> IVGGYTCGANTVPYQVSL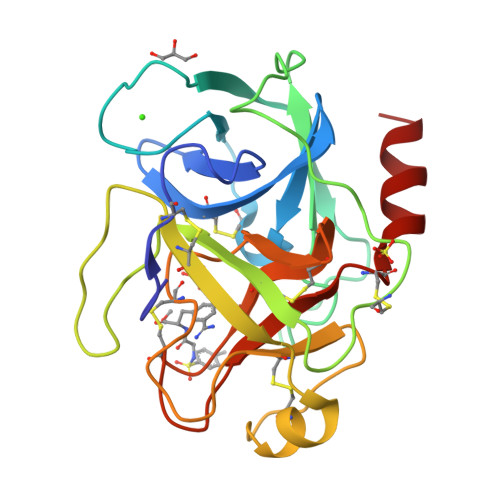NSGYHFCGGSLINSQWVVSAAHCYKSGIQVRLGEDNINVVEGNEQFISASKSIVHPSYNSETYNNDIMLIKLKSAASLNSRVASISLPTSCASAGTQCLISGWGNTKSSGTSYPDVLKCLKAPILSDSSCKSASSFIITSNMFCAGYLEGGKDACQGDSGGPVVCSGKLQGIVSWGSGCAQKNKPGFYTKVCNYVSWIKQTIASN>MKEFTINNYLEDIRKKVPAYDLMLEIIFNSILKIETDISQIKNILSIGGQSFEVKNLSKIYNNSKITIIEPSEIMLNIVKNECKNLKNLEYIYDKFENYKDNKNFELCLCLLVLQFIEEPQSFLEKIYNSLDSNGLLIISIFSNKQLTYWKEFALSRGAKKEQVEKTFNNQSEVMNILSPEYV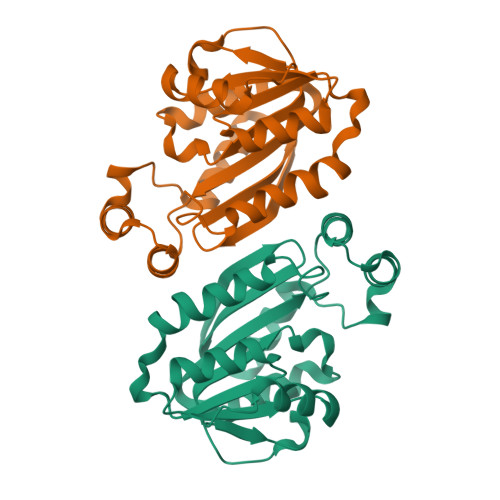EGLLKESGFSKIERICEVLSTDMWVVRK[8x]>TRDQNGTWEMESNENFEGYMKALDIDFATRKIAVRLTQTKVIDQDGDNFKTKTTSTFHHHRNYDVDFTVGVEFDEYTKSLDNRHVKALVTWEGDVLVCV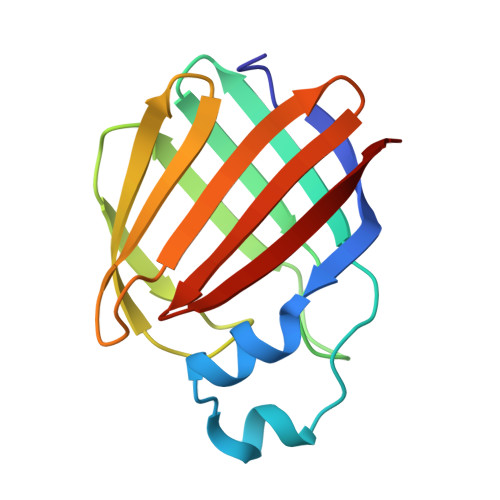QKGEKENRGWKQWIEGDKLYLELTCGDQVCRQVFKKK[2x]>GPLGSVEEIRLPRAGGPLGLSIVGGSDHSSHPFGVQEPGVFISKVLPRGLAARSGLRVGDRILAVNGQDVR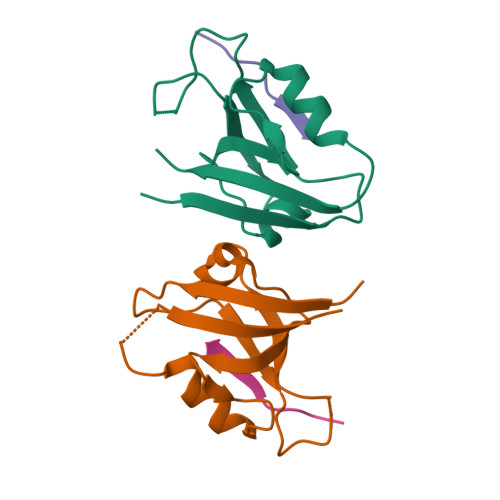DATHQEAVSALLRPCLELSLLVRRD[2x];>[2x]PAWDETNL> MHHHHHHMVDEILKLKKEKGYIILAHNYQIPELQDIADFVGDSLQLARKAMELSEKKILFLGVDFMAELVKILNPDKKVIVPDRSATCPMLNRLTPEIIREYREKFPDAPVVLYVNSTSECKTLADVICTSANAVEVVKKLDSSVVIFGPDRNLGEYVAEKTGKKVITIPENGHCPVHQFNAESIDAVRKKYPDAKV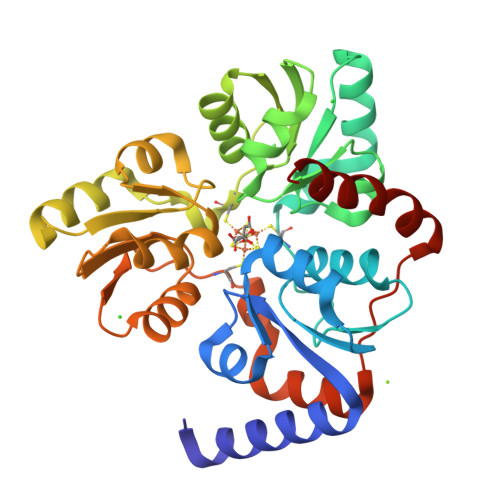IVHPECPKPVRDKADYVGSTGQMEKIPERDPSRIFVIGTEIGMIHKLKKKFPDREFVPLEMAVCVNMKKNTLENTLHALQTESFEVILPKEVIEKAKKPILRMFELMG>MHHHHHHPEIVDTCSLASPASVCRTKHLHLRCSVDFTRRTLTGTAALTVQSQEDNLRSLVLDTKDLTIEKVVINGQEVKYALGERQSYKGSPMEISLPIALSKNQEIVIEISFETSPKSSALQWLTPEQT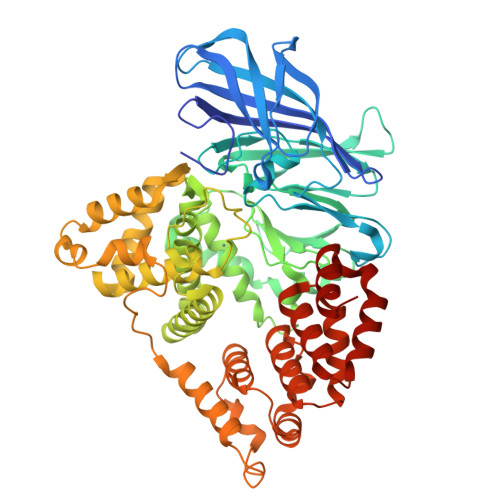SGKEHPYLFSQCQAIHCRAILPCQDTPSVKLTYTAEVSVPKELVALMSAIRDGETPDPEDPSRKIYKFIQKVPIPCYLIALVVGALESRQIGPRTLVWSEKEQVEKSAYEFSETESMLKIAEDLGGPYVWGQYDLLVLPPSFPYGGMENPCLTFVTPTLLAGDKSLSNVIAHEISHSWTGNLVTNKTWDHFWLNEGHTVYLERHICGRLFGEKFRHFNALGGWGELQNSVKTFGETHPFTKLVVDLTDIDPDVAYSSVPYEKGFALLFYLEQLLGGPEIFLGFLKAYVEKFSYKSITTDDWKDFLYSYFKDKVDVLNQVDWNAWLYSPGLPPIKPNYDMTLTNACIALSQRWITAKEDDLNSFNATDLKDLSSHQLNEFLAQTLQRAPLPLGHIKRMQEVYNFNAINNSEIRFRWLRLCIQSKWEDAIPLALKMATEQGAMKFTRPLFKDLAAFDKSHDQAVRTYQEHKASMHPVTAMLVGKDLKVD[3x]2-methyl-5-(trifluoromethyl)-1~{H}-pyrrole-3-carboxylic acid | C7 H6 F3 N O2 | 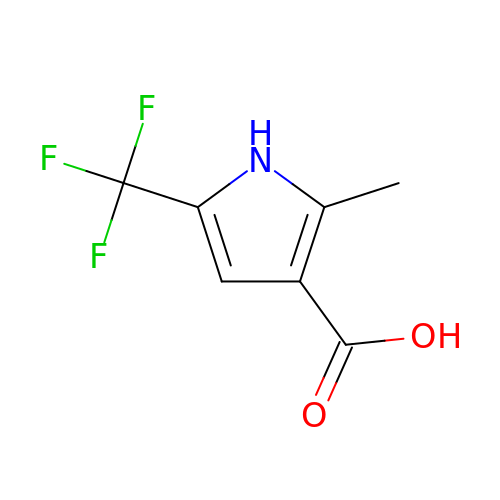FZYQYTJVKWEWQJ-UHFFFAOYSA-N>GPHMDLRPVVIDGSNVAMSHGNKEVFSCRGILLAVNWFLERGHTDITVFVPSWRKEQPRPDVPITDQHILRELEKKKIL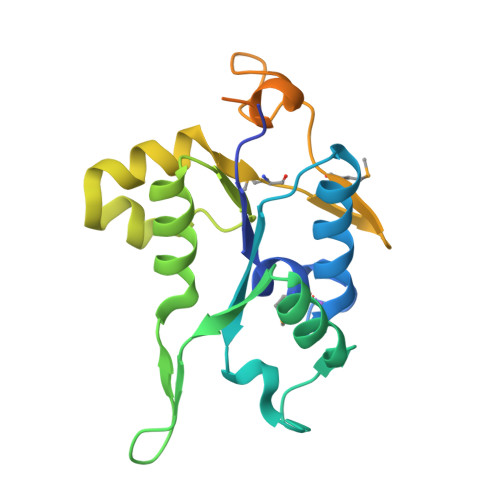VFTPSRRVGGKRVVCYDDRFIVKLAFESDGVVVSNDTYRDLQGERQEWKRFIEERLLMYSFVNDKFMPPDDPLGRHGPSLDNFLRKKPLPSEHRKQPCPYGKKCTYGIKCRFFHPERPSRPQRSVADELRA[4x]> MPKRTDIKSILILGAGPIVIGQACEFDYSGAQACKALREEGYRVINVNSNPATIMTDPEMADATYIEPIHWEVVRKIIEKERPDAVLPTMGGQTALNCALELERQGVLEEFGVTMIGATADAIDKAEDRRRFDVAMKKIGLETARSGIAHTMEEALAVAADVGFPCIIRPSFTMGGSGGGIAYNREEFEEICARGLDLSPTKELLIDESLIGWKEYEMEVVRDKNDNCIIVCSIENFDAMGIHTGDSITVAPAQTLTDKEYQIMRNASMAVLREIGVETGGSNVQFAVNPKNGRLIVIEMNPRVSRSSALASKATGFPIAKVAAKLAVGYTLDELMNDITGGRTPASFEPSIDYVVTKIPRFNFEKFAGANDRLTTQMKSVGEVMAIGRTQQESLQKALRGLEVGATGFDPKVSLDDPEALTKIRRELKDAGADRIWYIADAFRAGLSVDGVFNLTNIDRWFLVQIEELVRLEEKVAEVGITGLNADFLRQLKRKGFADARLAKLAGVREAEIRKLRDQYDLHPVYKRVDTCAAEFATDTAYMYSTYEEECEANPSTDREKIMVLGGGPNRIGQGIEFDYCCVHASLALREDGYETIMVNCNPETVSTDYDTSDRLYFEPVTLEDVLEIVRIEKPKGVIVQYGGQTPLKLARALEAAGVPVIGTSPDAIDRAEDRERFQHAVERLKLKQPANATVTAIEMAVEKAKEIGYPLVVRPSYVLGGRAMEIVYDEADLRRYFQTAVSVSNDAPVLLDHFLDDAVEVDVDAICDGEMVLIGGIMEHIEQAGVHSGDSACSLPAYTLSQEIQDVMRQQVQKLAFELQVRGLMNVQFAVKNNEVYLIEVNPRAARTVPFVSKATGVPLAKVAARVMAGKSLAEQGVTKEVIPPYYSVKEVVLPFNKFPGVDPLLGPEMRSTGEVMGVGRTFAEAFAKAQLGSNSTMKKHGRALLSVREGDKERVVDLAAKLLKQGFELDATHGTAIVLGEAGINPRLVNKVHEGRPHIQDRIKNGEYTYIINTTSGRRAIEDSRV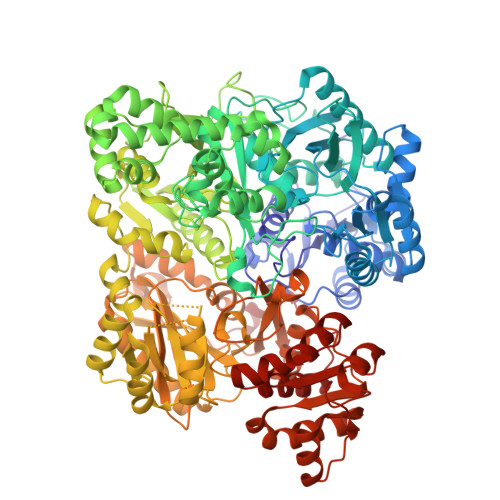IRRSALQYKVHYDTTLNGGFATAMALNADATEKVISVQEMHAQIK>[2x]MKDWLFRIATCSIMTFSSLAAAQAEPLDVVATFSIIGDFAAKVGGDRIRLNVLVGPDSDTHVYEPRPADAIALAGADVVLTNGLEFEGFLTRLIAASGTDAAVATLTDGVETMEEPGGGHYHYIDGKAVFHAGAHDPHAWQAVPNAKVYVQNIAAAFCAADAEGCAAYQANAARYIGELDALDTEIRAAIAALPQDRRTVVVAHNAFRYFEAAYGVHFLSPAAAADVAGLIREIRARNASAIFAENISDTRLLEQIAREAGLPLAGTLYSDALSGPDGPASNYIAMMRHNAGAIAAALAAR

In addition to dimeric membrane permease and cytosolic ATPase proteins, bacterial ABC transporters rely on periplasmic (Gram-negative) or cell surface (Gram-positive) solute binding proteins (SBP). The SBP is essential to bind the substrate with high affinity and specificity and deliver it to the membrane permease for transport into the cell. SBPs have been categorized according to structure and substrate specificity, with members of group A-I mediating transport of zinc, manganese, or iron. Secondly, AztC (residues 222–229) referred to as the Z-loop must be displaced away from the zinc binding site in order for the complex to form.

In order to determine what structural features of ΔZ-Loop AztC might mediate its more rapid transfer kinetics, a crystal structure was determined for this mutant. The overall structure is very similar to that of the holo WT, with rmsd = 0.26–0.30 Å across all atoms depending on which chains are aligned. The zinc binding site is also completely superimposable. Residues 117–133 (the D-Loop) could not be modeled into either chain of the ΔZ-Loop AztC structure due to a lack of electron density. Residues 222–229 (the Z-Loop) are absent, leaving a run of four Ala residues. Electron density in this region is also somewhat weak, indicating some flexibility. The deletion shortens the loop between helices α7 and α8, preventing closure of the loop over the zinc binding site as is observed for the WT. The lack of any other significant structure changes as a result of the deletion suggest that this is the primary reason for the increase in zinc dissociation rate and transfer rate from AztD. Deletion of the Z-Loop in AztC causes a roughly 6-fold increase in the dissociation rate of zinc relative to WT, suggesting that closure of this loop over the zinc slows its dissociation. Here we demonstrate that the rate of transfer from WT AztD to ΔZ-Loop AztC is increased approximately two-fold relative to WT AztC under the same conditions.>[3x]MDSSEVVKVKQASIPAPGSILSQPNTEQSPAIVLPFQFEATTFG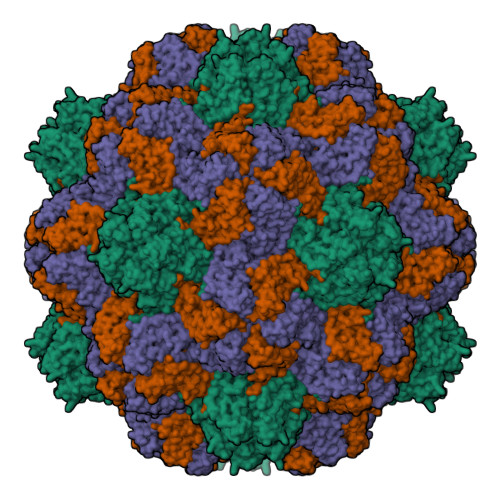TAETAAQVSLQTADPITKLTAPYRHAQIVECKAILTPTDLAVSNPLTVYLAWVPANSPATPTQILRVYGGQSFVLGGAISAAKTIEVPLNLDSVNRMLKDSVTYTDTPKLLAYSRAPTNPSKIPTASIQISGRIRLSKPMLIAN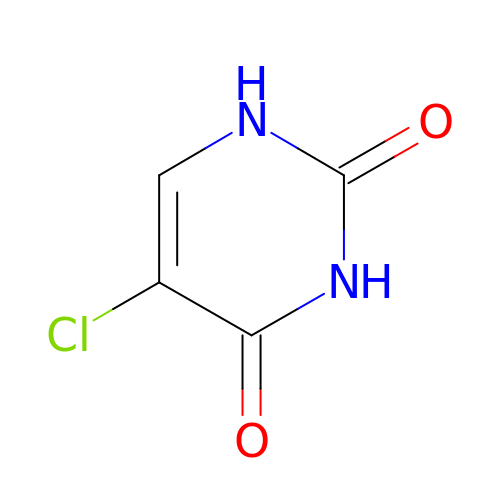5-chloropyrimidine-2,4(1H,3H)-dione | C4 H3 Cl N2 O2 | ZFTBZKVVGZNMJR-UHFFFAOYSA-N> SKYSAPDFDEDDQQMQQQTQQKQQQTQPSKVTFQQPSTKLTKPKFTANLDNFDSDSETSSGDENQDEMVPQKKTPFIKRVSNRESGLFDTPSVVPMSEKIETTPSKIARVSEPTSQSSRMSNNALKFSTFNPQQQQLQSSRFKSTGLSILSNPVKNLIQSDVNNEQSMFSNTTTTSTTRIQPLPSQQHLVQPIPTTISLNKNYFSKVRIDPQVYDRIVPKEESITNQYRMKNERLNHSTQDVSLFMRRSFRVGWAPGGKLISITKSSFKNLLIKKLPTDTKEDKKESIIKFLKNHHSHSSLVPENLKSIGWFSISNVQEQIESQLTLNVPSSQSVYYNRIWSLISNLWGNVLKGNGSKYINTNYSEDTIRKLNLNQWLKDVIAPLLRDEMDSLRKKTNSNYLEQIFSYLSAKQIKEASDLANENKDFRLATMMSQIWSSSESGKELILKQLTTYHSNGSDEFINEKRLEILHLIAGSVNKIYKNLNDWIRCFAVSFWFKYSLEYSIEDSVENFERSFNAHRSVYPLPPYLIKSTSTNSKQIEE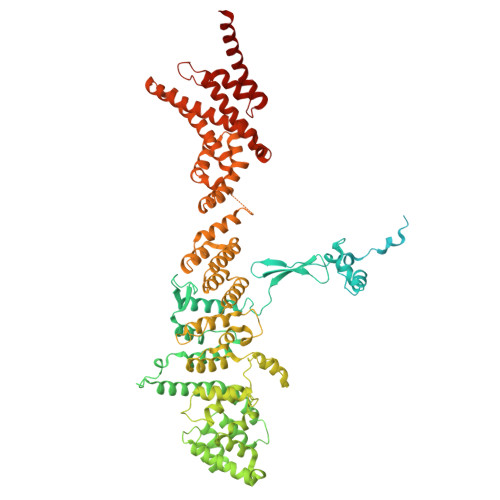QQHYYDICFLLLKLFAVNRGSSHFDKFKNIFYPENIGQDLLDYHLSWNLYTVLKSIPSLNKQPDLVNASNLHSSFALQLERLGLWQWSIYVLLHTPDQSNHVREEAVKSLIARAAPVITSEDRVFLTTKLHIPEIWIDEAKAWYSGYDCNNDIYDQIDALFKSYQYTKIHDIIFSNIGPNYIIQKRYHSLKDLLIRLEPHSSFISTWRYGGSIFLEFADICIQYKEILSQLSNTAEEIQRTKYYVNLKDITTRIVNILSDISKITQSSEIKNTSASYKQSLSFMSEALITKASLLRDLPESIVKLVSTNNLVSTLNSLPLTQDYRSKNLESLTDQIQDTLLNSIYQ> EFGDLSGIISRDQFYKMLKHMNDNDCHAVGFFTYDAFITAAKSFPSFGNTGDLAMRKKEIAAFFGQTSHETTGGWSGAPDGANTWGYCYKEEIDKS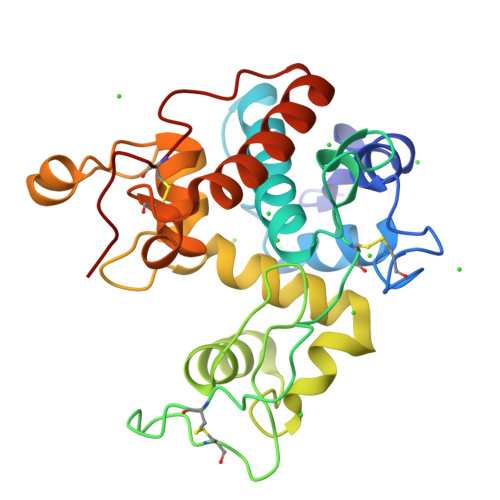DPHCDSNNLEWPCAPGKFYYGRGPMMLSWNYNYGPCGRDLGLELLKNPDVASSDPVIAFKTAIWFWMTPQAPKPSCHDVITDQWEPSAADISAGRLPGYGVITNIINGGLECAGRDVAKVQDRISFYTRYCGMFGVDPGSNIDCDNQRPFN> HMDTSILNLRYESNHLIDLSRYASKINIGSKVNFDPIDKNQIQLFNLESSKIEVILKNAIVYNSMYENFSTSFWIRIPKYFNSISLNNEYTIINCMENNSGWKVSLNYGEIIWTLQDTQEIKQRVVFKYSQMINISDYINRWIFVTITNNRLNNSKIYINGRLIDQKPISNLGNIHASNNIMFKLDGCRDTHRYIWIKYFNLFDKELNEKEIKDLYDNQSNSGILKDFWGDYLQYDKPYYMLNLYDPNKYVDV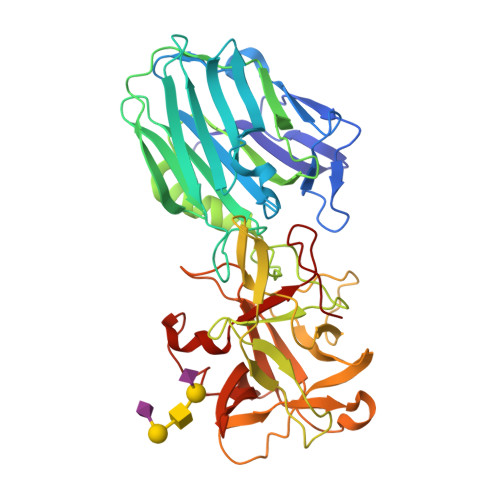NNVGIRGYMYLKGPRGSVMTTNIYLNSSLYRGTKFIIKKYASGNKDNIVRNNDRVYINVVVKNKEYRLATNASQAGVEKILSALEIPDVGNLSQVVVMKSKNDQGITNKCKMNLQDNNGNDIGFIGFHQFNNIAKLVASNWYNRQIERSSRTLGCSWEFIPVDDGWGERPLQ> GSPEFVQGNTDEAQEE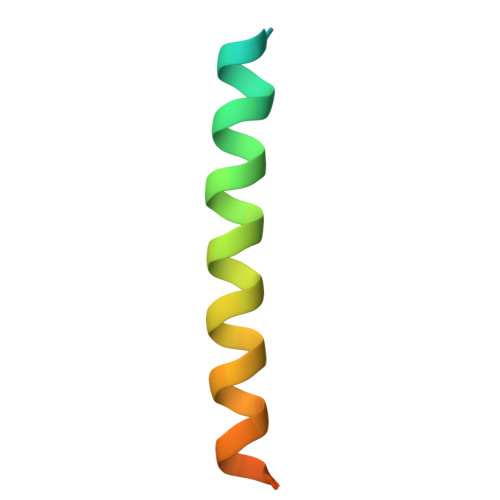LAWKIAKMIVSDVMQQAQYDQPLEKSTKL> APLAAMDECADEGGRPQRCMPEFVNAAFNVTVVATNTCGTPPEEYCVQTGVTGVTKSCHLCDAGQQHLQHGAAFLTDYNNQADTTWWQSQTMLAGVQYPNSINLTLHLGKAFDITYVRLKFHTSRPESFAIYKRTREDGPWIPYQYYSGSCENTYSKANRGFIRTGGDEQQALCTDEFSDISPLTGGNVAFSTLEGRPSAYNFDNSPVLQEWVTATDIRV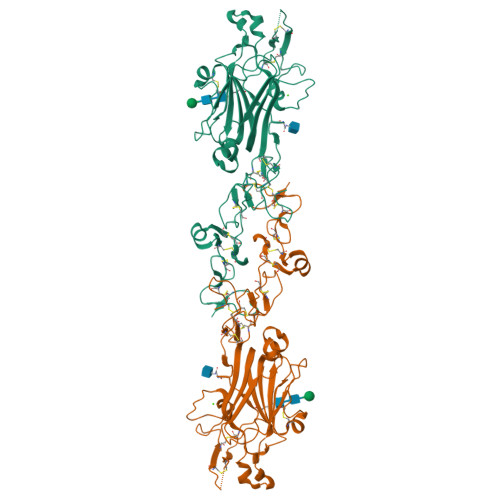TLNRLNTFGDEVFNEPKVLKSYYYAISDFAVGGRCKCNGHASECVKNEFDKLMCNCKHNTYGVDCEKCLPFFNDRPWRRATAESASECLPCDCNGRSQECYFDPELYRSTGHGGHCTNCRDNTDGAKCERCRENFFRLGNTEACSPAAAHHHHHH RIBULOSE-1,5-DIPHOSPHATE | 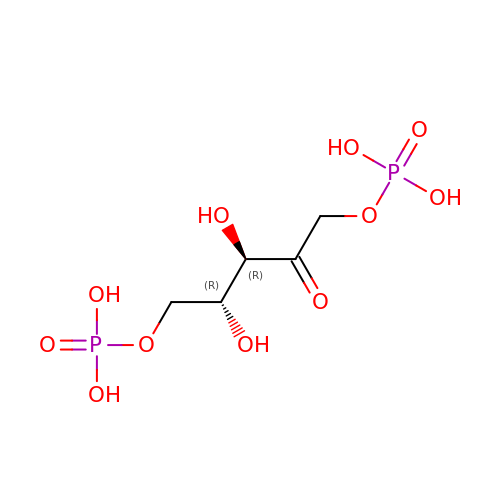C5 H12 O11 P2 | YAHZABJORDUQGO-NQXXGFSBSA-N(S)-2-amino-3-(2-(2-carboxyethyl)-5-chloro-4-nitrophenyl)propionic acid | C12 H13 Cl N2 O6 | 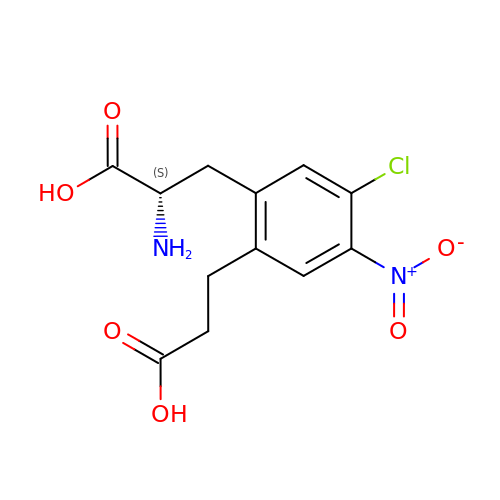DRCLPFURMHGQPC-VIFPVBQESA-N>[2x]MAGNDSNLIWLDLEMTGLEPVEDVILEIAIIITDSELNILAQGPIFAISQTDDVLDNMNPWCIEHHGKSGLTQRCRDSEVSLAHATKESLAFVQEWVP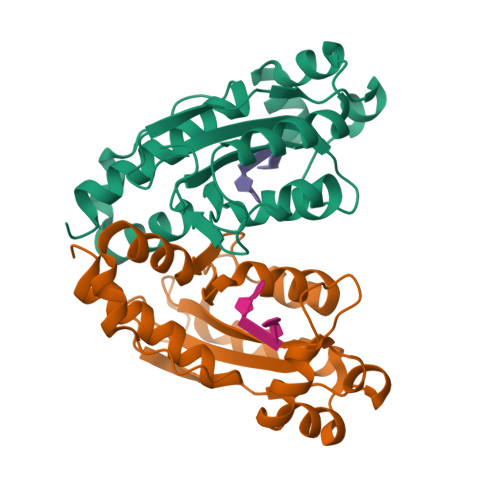QGKSPMCGNSIGQDRRFINKYMPDFEDHFHYRNLDVSTIKELAKRWKPEVLESVVKTGAHLALDAIKESIAELKVYRELFFKL> MEADARSIYVGNVDYG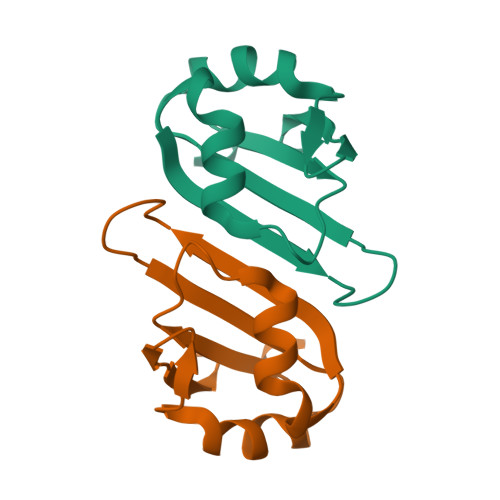ATAEELEAHFHGCGSVNRVTILCDKFSGHPKGFAYIEFSDKESVRTSLALDESLFRGRQIKVIPKRTNRPGILEHHHHHH> MSFVAYEELIKEGDTAILSLGHGAMVAVRVQRGAQTQTRHGVLRHSVDLIGRPFGSKVTCGRGGWVYVLHPTPELWTLNLPHRTQILYSTDIALITMMLELRPGSVVCESGTGSGSVSHAIIRTIAPTGHLHTVEFHQQRAEKAREEFQEHRVGRWVTVRTQDVCRSGFGVSHVADAVFLDIPSPWEAVGHAWDALKVEGGRFCSFSPCIEQVQRTCQALAARGFSELSTLEVLPQVYNVRTVSLPPPDLGTGTDGPAGSDTSPFRSGTPMKEAVGHTGYLTFATKT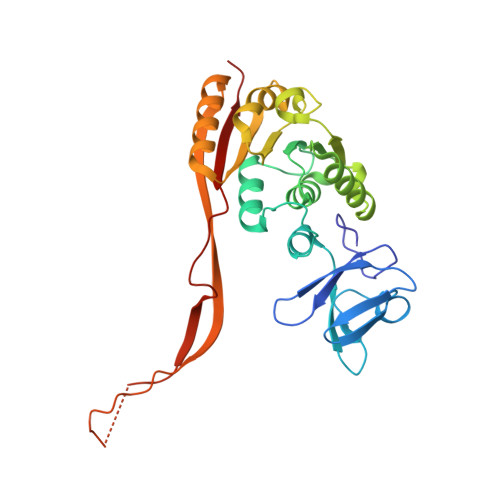PG>KPQVTILATGGTIAGSGESSKTSSYSAGAVTVDKLLAAVPAINDLATIKGEQISSIGSQEMTGKVWLKLAKR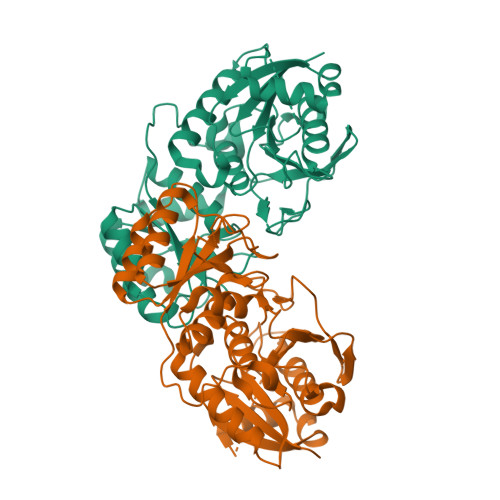VNELLAQKETEAVIITHGTDTMEETAFFLNLTVKSQKPVVLVGAMRPGSSMSADGPMNLYNAVNVAINKASTNKGVVIVMNDEIHAAREATKLNTTAVNAFASPNTGKIGTVYYGKVEYFTQSVRPHTLASEFDISKIEELPRVDILYAHPDDTDVLVNAALQAGAKGIIHAGMGNGNPFPLTQNALEKAAKSGVVVARSSRVGSGSTTQEAEVDDKKLGFVATESLNPQKARVLLMLALTKTSDREAIQKIFSTY[2x]>[2x]PIFEARVKVGISSSWVTSRKVSWRDAIAQIESDRIVVKYLKMGEVVGEDSFPFSALIDLGVRIPDELKLNPEKDHFGIKFYIPGRGELLVIFTIEENLLIYDEKKFSEFVHKVFEVLINGKTVMLQLARIIGGAVNMESKWEEGWLRV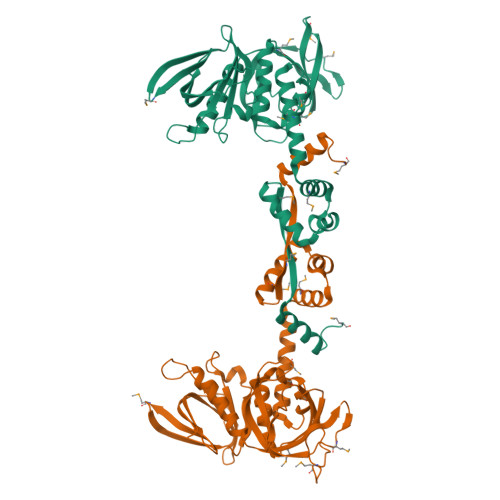IKVKSARTQKTERSIVVIIKDKRPVSIFSDLEDIEIEEVDMNGKRVRAWKIRHFHIDQSVTSYLYIPDKQTQLYVLRYLLKYNPAIMEFIMKVSDDFPTLKSEFQEIMEKEIKELEALDEMEKQILVALYSGINPLELHQFLGVSEKEIEEIYDRMIDKGLLKIVMIRKIVDLTNEGRKIVNKLLKYGLVSM> IVDTCSLASPASVCRTKHLHLRCSVDFTRRTLTGTAALTVQSQEDNLRSLVLDTKDLTIEKVVINGQEVKYALGERQSYKGSPMEISLPIALSKNQEIVIEISFETSPKSSALQWLTPEQTSGKEHPYLFSQCQAIHCRAILPCQDTPSVKLTYTAEVSVPKELVALMSAIRDGETPDPEDPSRKIYKFIQKVPIP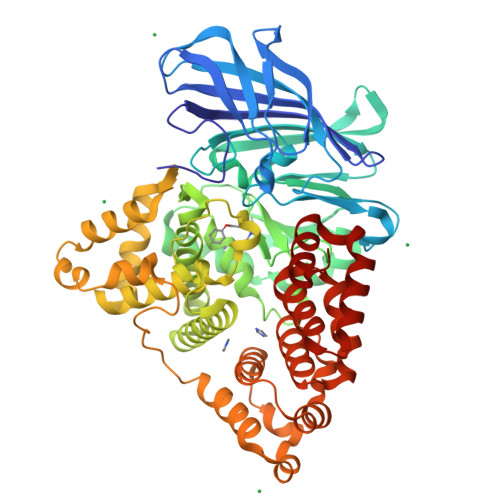CYLIALVVGALESRQIGPRTLVWSEKEQVEKSAYEFSETESMLKIAEDLGGPYVWGQYDLLVLPPSFPYGGMENPCLTFVTPTLLAGDKSLSNVIAHEISHSWTGNLVTNKTWDHFWLNEGHTVYLERHICGRLFGEKFRHFNALGGWGELQNSVKTFGETHPFTKLVVDLTDIDPDVAYSSVPYEKGFALLFYLEQLLGGPEIFLGFLKAYVEKFSYKSITTDDWKDFLYSYFKDKVDVLNQVDWNAWLYSPGLPPIKPNYDMTLTNACIALSQRWITAKEDDLNSFNATDLKDLSSHQLNEFLAQTLQRAPLPLGHIKRMQEVYNFNAINNSEIRFRWLRLCIQSKWEDAIPLALKMATEQGRMKFTRPLFKDLAAFDKSHDQAVRTYQEHKASMHPVTAMLVGKDLKVD>[2x]PDISAKDLRNIMYDHL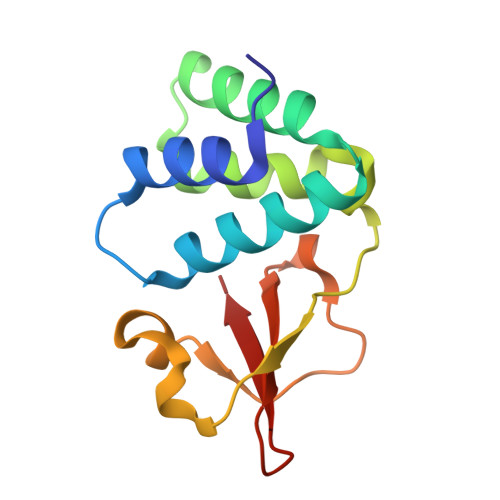PGFGTAFHQLVQVICKLGKDSNSLDIIHAEFQASLAEGDSPQCALAQITKRVPIFQDAAPPVIHIRSRGDIPRACQKSLRPVPPSPKIDRGWVCVFQLQDGKTLGLKI>SATRANKDIFTLFDKKGQGAIAKDSLGDYLRAIGYNPTNQLVQDIINADSSLRDASSLTLDQITGLIEVNEKELDATTKAKTEDFVKAFQVFDKESTGKVSVGDLRYMLTGLGEKLTDAEVDELLKGVEVDSNGEIDYKK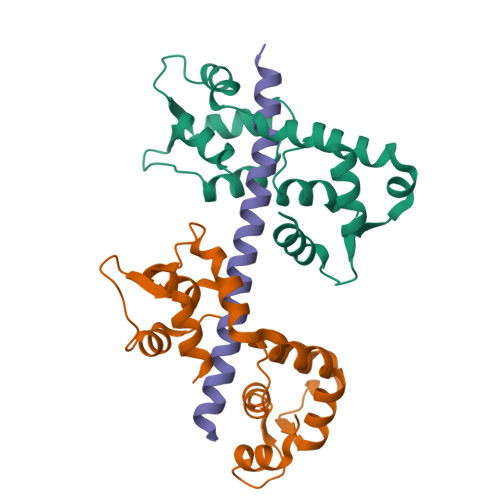FIEDVLRQ[2x];> QISQAIKYLQNNIKGFIIRQRVNDEMKVNCATLLQAAYRGHSIRANVF> MAEQVALSRTQVCGILREELFQGDAFHQSDTHIFIIMGASGDLAKKKIYPTIWWLFRDGLLPENTFIVGYARSRLTVADIRKQSEPFFKATPEEKLKLEDFFARNSYVAGQYDDAASYQRLNSHMNALHLGSQANRLFYLALPPTVYEAVTKNIHESCMSQ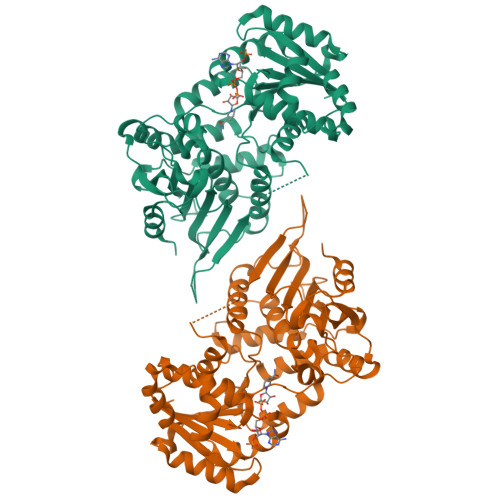IGWNRIIVEKPFGRDLQSSDRLSNHISSLFREDQIYRIDHYLGKEMVQNLMVLRFANRIFGPIWNRDNIACVILTFKEPFGTEGRGGYFDEFGIIRDVMQNHLLQMLCLVAMEKPASTNSDDVRDEKVKVLKCISEVQANNVVLGQYVGNPDGEGEATKGYLDDPTVPRGSTTATFAAVVLYVENERWDGVPFILRCGKALNERKAEVRLQFHDVAGDIFHQQCKRNELVIRVQLNEAVYTKMMTKKPGMFFNPEESELDLTYGNRYKNVKLPDAYERLILDVFCGSQMHFVRSDELREAWRIFTPLLHQIELEKPKPIPYIYGSRGPTEADELMKRVGFQYEGTYKWVNPHKL> MTTLADVKKRIGLKDEKQDEQLEEIIKSCESQLLSMLPIEVEQIPERFSYMIKEVAVKRYNRIGAEGMTSEAVDGRSNAYELN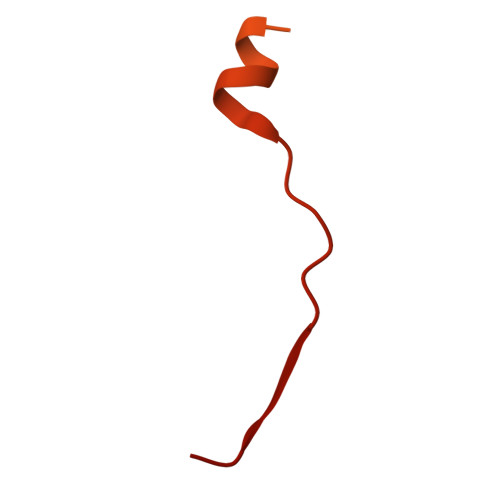DFKEYEAIIDNYFNARTRTKKGRAVFF> MFGYWDPLYFIIVFIIGLILAYLLNLWAKKSGMGTREVGEGTKIFISGEDPEKVIPGFEHLEGYYTGRNTMWGLVNGVKKFFATLKNDHTGL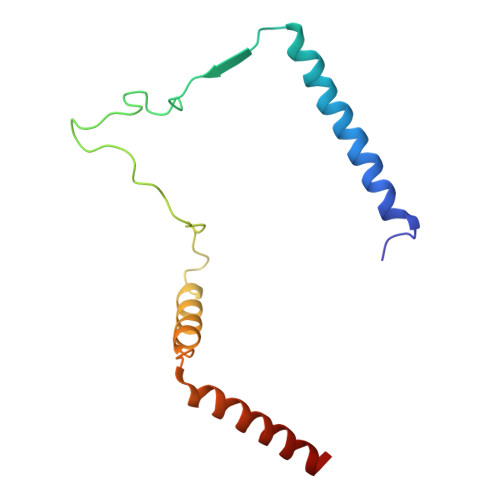LPDYVSYLLMTTAFILVILLLRG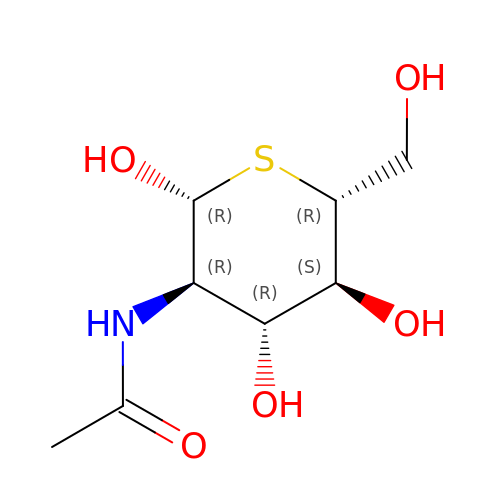2-acetamido-2-deoxy-5-thio-beta-D-glucopyranose | C8 H15 N O5 S | DYCCLPFFILCZGU-FMDGEEDCSA-N>[2x]GNSDDARTSIEQRSNAVSQVLLGIFSYVRWPKEPAVLQLCVVGPTEYADGLLRGMVQANGRRVHAERRAVDNPDLGTLCNVIYLGVVDERERQQVFRSLAGHPVLSISERGTECSVGSMFCLNVGGPRITFEANLDSIARSGVRVHPSVLKLARRQATP

The YfiBNR system contains three protein members and modulates intracellular c-di-GMP levels in response to signals received in the periplasm. YfiN is repressed by specific interaction between its periplasmic PAS domain and the periplasmic protein YfiR. YfiB is an OmpA/Pal-like outer-membrane lipoprotein that can activate YfiN by sequestering YfiR in an unknown manner. Previous studies suggested that in response to cell stress, YfiB in the outer membrane sequesters the periplasmic protein YfiR, releasing its inhibition of YfiN on the inner membrane and thus inducing the diguanylate cyclase activity of YfiN to allow c-di-GMP production.

Moreover, we found that Vitamin B6 (VB6) or L-Trp can bind YfiR with an affinity in the ten millimolar range. Structural analyses revealed that the VB6 and L-Trp molecules are bound at the periphery of the YfiR dimer, but not at the dimer interface. Interestingly, VB6 and L-Trp were found to occupy the same hydrophobic pocket, formed by L166/I169/V176/P178/L181 of YfiR, which is also a binding pocket for F57 of YfiB, as observed in the YfiB-YfiR complex. To answer the question whether competition of VB6 or L-Trp for the YfiB F57-binding pocket of YfiR plays an essential role in inhibiting biofilm formation, we measured the binding affinities of VB6 and L-Trp for YfiR via BIAcore experiments. The results showed relatively weak Kd values of 35.2 mmol/L and 76.9 mmol/L for VB6 and L-Trp, respectively. The over-expression of YfiBL43P induced strong surface attachment and much slower growth of the yfiB-L43P strain, and as expected, a certain amount of VB6 or L-Trp (4–6 mmol/L for VB6 and 6–10 mmol/L for L-Trp) could reduce the surface attachment. In E. coli, mutants with decreased tryptophan synthesis show greater biofilm formation, and matured biofilm is degraded by L-tryptophan addition. Based on our results, we concluded that VB6 or L-Trp can bind to YfiR, however, VB6 or L-Trp alone may have little effects in interrupting the YfiB-YfiR interaction, the mechanism by which VB6 or L-Trp inhibits biofilm formation remains unclear and requires further investigation.> LTQVVHSAGRRFIVS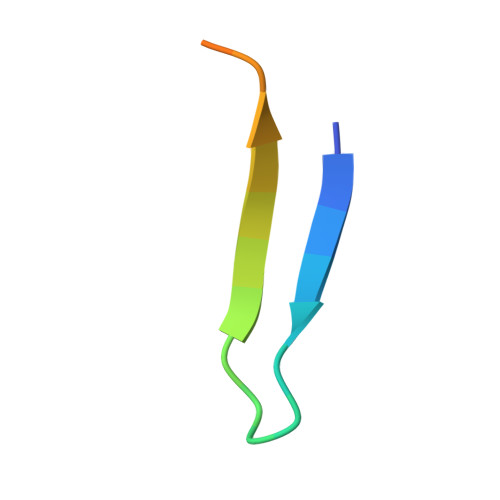PVPESRLR> MRFPSIFTAVLFAASSALAAPVNTTTEDETAQIPAEAVIGYSDLEGDFDVAVLPFSNSTNNGLLFINTTIASIAAKEEGVSLEKREAEAYVEFQINVDLQARYQSVDGFGCSQAFQRAEDIFGKYGLSPKNQSYVLDLMYSEERGAGFTILRNGIGSSNSSTSNLMNSIEPFSPGSPSSTPNYTWDHYNSGQFPLSQQARARGLPYIYADAWSAPGYMKTNQDENWSGFLCGIEGETCPSGDWRQAYADYLVQYVKFYAESGVPVTHLGFLNEPQEVVSYASMGSNGTQAAEFVKILGQTLEREGIDIELTCCDGVGWSEQEAMIPGLQVVGPDGKSAEDYLSVVTGHGYSSAPTFPLSTKRRTWLTEWTDLSGAFTPYTFFADGGAGEGMTWANHIQTAFVNANVSAFIYWIGAENSTTNSGMINLINDEVIPSK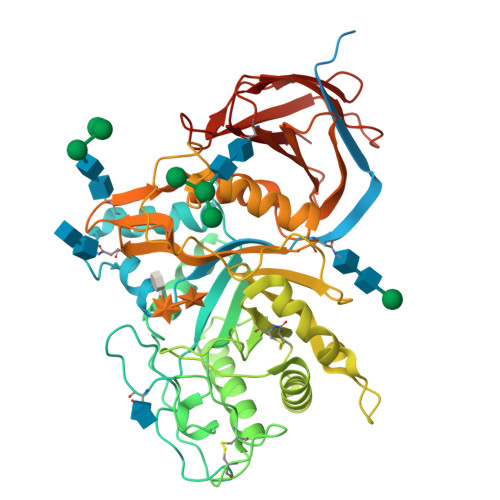RFWSMASFSKFVRPNAQRVKATSSDASVTVSAFENTNGVVAIQVINNGTSAASLTIDLGKTHKEVKKVVPWVTSNDYDLEEMSEIDVKHNSFLASVPARSLTSFVTECE> TQKPSLYRVLILNDDYTPMEFVVYVLERFFNKSREDATRIMLHVHQNGVGVCGVYTYEVAETKVAQVIDSARRHQHPLQC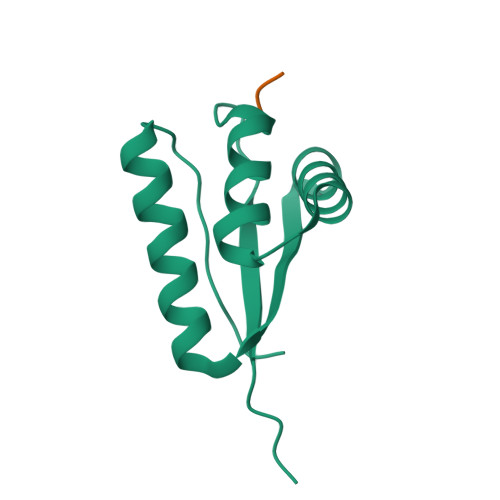TMEKD;> LLL> MSFLISFDKSKKHPAHLQLANNLKIALALEYASKNLKPEVD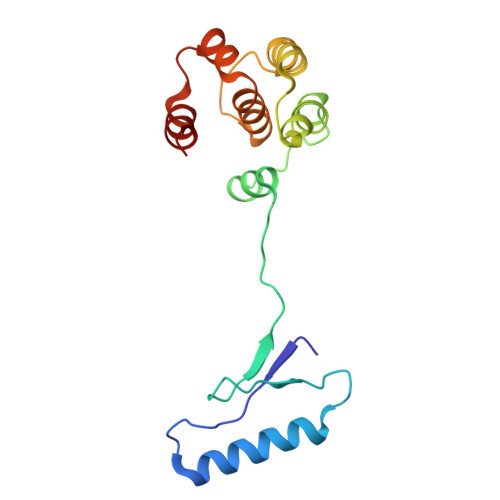NDNAAMELRNTKEPFLLFDANAILRYVMDDFEGQTSDKYQFALASLQNLLYHKELPQQHVEVLTNKAIENYLVELKEPLTTTDLILFANVYALNSSLVHSKFPELPSKVHNAVALAKKH> MAATAAEAVASGSGEPREEAGALGPAWDESQLRSYSFPTRPIPRLSQSDPRAEELIENEEPVVLTDTNLVYPALKWDLEYLQENIGNGDFSVYSASTHKFLYYDEKKMANFQNFKPRSNREEMKFHEFVEKLQDIQQRGGEERLYLQQTLNDTVGRKIVMDFLGFNWNWINKQQGKRGWGQLTSNLLLIGMEGNVTPAHYDEQQNFFAQIKGYKRCILFPPDQFECLYPYPVHHPCDRQSQVDFDNPDYERFPNFQNVVGYETVVGPGDVLYIPMYWWHHIESLLNGGITITVNFWYKGAPTPKRIEYPLKAHQKVAIMRNIEKMLGEALGNPQEVGPLLNTMIKGRYN;> HLEVVKLLLEAGADVNAQDK

2-Oxoglutarate (2OG) and Fe(II)-dependent oxygenases couple substrate oxidation with 2OG decarboxylation to give succinate and CO2; they have important functions in human biology, e.g., in hypoxia signaling, extracellular matrix biosynthesis, lipid metabolism, and DNA/RNA damage repair. The human 2OG oxygenases studied, factor inhibiting hypoxia-inducible transcription factor HIF-α (FIH) and aspartate/asparagine-β-hydroxylase (AspH), catalyze C3 hydroxylations of Asp/Asn-residues. Like AspH, human factor inhibiting the hypoxia-inducible transcription factor HIF-α (FIH) catalyzes the post-translational oxidation of Asp- and Asn-residues in a 2OG-dependent manner, however, to give the β-threo hydroxylated product. FIH was initially identified as catalyzing hydroxylation of an Asn-residue in the C-terminal transactivation domain of HIF-α isoforms (Asn803 in HIF-1α), a reaction that suppresses HIF-mediated transcription.

High levels of FIH substrate hydroxylation were observed for 3-methyl-2OG and 4-methyl-2OG, both of which are natural products, regardless of the substrate, indicating that these 2OG derivatives can efficiently replace 2OG (entries 2 and 13). NMR studies reveal that FIH converts 1 and 12 into 2-methylsuccinate with a similar efficiency to which it converts 2OG into succinate. Notably, 3-methyl-2OG is an efficient cosubstrate for both FIH and AspH (entry 2), whereas its isomer 4-methyl-2OG is apparently more efficient in maintaining FIH compared with AspH activity (entry 13). The FIH Kmapp-value for 4-methyl-2OG is similar to that of 2OG, indicating a similar affinity; by contrast, the FIH Kmapp-value for 1, the 3-methyl regioisomer of 12, is higher. The observation that the conformations of C3- and C4-alkyl 2OG derivatives are very similar to that of 2OG in complex with FIH is in agreement with their similar Kmapp-values. Although the C3/C4-alkyl 2OG derivatives were used as racemic mixtures, the crystallographic analyses reveal that, at least predominantly, the (S)-enantiomers of the 2OG derivatives bind to FIH, potentially owing to their ability to engage in more efficient hydrophobic interactions with the hydrophobic Leu186 and Leu188 sidechains. The increase in length of the 2OG C3/C4-substituent from methyl via ethyl to propyl appears to correlate with enhanced FIH inhibition. Thus, although the C3/C4 methyl-substituted 2OG derivatives 1 and 12 do not inhibit FIH (entries 2 and 7), 3-propyl-2OG inhibits FIH efficiently (IC50 ~2.7 μM; Table 3, entry 4).>SQIPASEQETLVRPKPLLLKLLKSVGAQKDTYTMKEVLFYLGQYIMTKRLYDAAQQHIVYCSNDLLGDLFGVPSFSVKE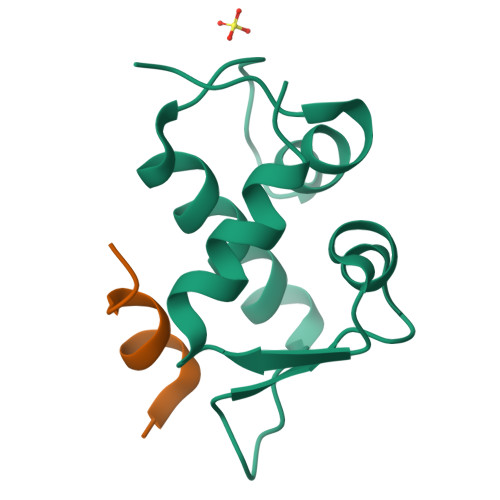HRKIYTMIYRNLVVVNQQESSDSGTSVSEN[2x];>[2x]SQETFSDLWKLLPEN>MNISDVAKITGLTSKAIRFYEEKGLVTPPMRSENGYRTYTQQHLNELTLLRQARQVGFNLEESGELVNLFNDPQRHSADVKRRTLEKVAEIERHIEELQSMRDQLLALANACPGDDSADCPIIENLSGCCHHRAG[2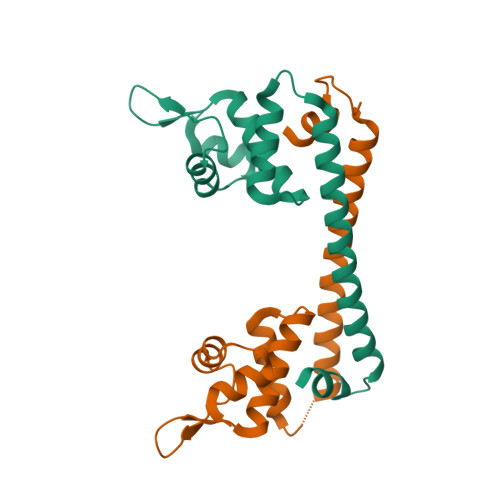x]p-sulfonatocalix[6]arene | C42 H30 O24 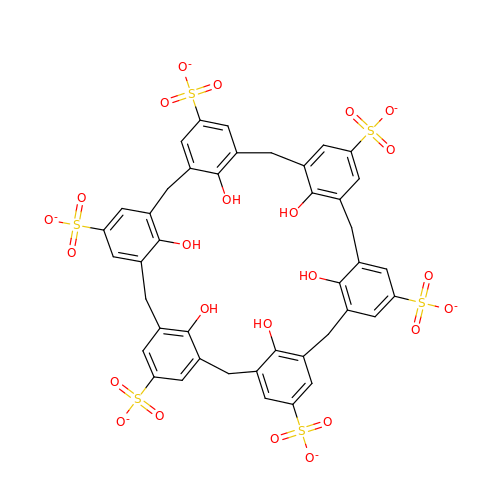S6 | BXOUPTJVBGEDIR-UHFFFAOYSA-H>AFFTTVIIPAIVGGIATGTAVGTVSGLLGWGLKQAEEANKTPDKPDKVWRIQAGKGFNEFPNKEYDLYKSLLSSKIDGGWDWGNAATHYWIKGGQWNKLEVDMKDAVGTYKLSGLRNFTGGDLDVNMQKATLRLGQFNGNSFTSYKDSADRTTRVDFNAKNILIDNFLEINNRVGSGAGRKASSTVLTLQASEGITSSKNAEISLYDGATLNLASNSVKLNGNVWMGRLQYVGAYLAPSYSTINTSKVTGEVNFNHLTVGDHNAAQAGIIASNKTHIGTLDLWQSAGLNIIAPPEGGYKDKPNNTPSQSGAKNDKQESSQNNSNTQVINPPNSTQKTEVQPTQVIDGPFAGGKDTVVNIDRINTKADGTIKVGGFKASLTTNAAHLNIGKGGVNLSNQASGRTLLVENLTGNITVDGPLRVNNQVGGYALAGSSANFEFKAGVDTKNGTATFNNDISLGRFVNLKVDAHTANFKGIDTGNGGFNTLDFSGVTNKVNINKLITASTNVAVKNFNINELIVKTNGVSVGEYTHFSEDIGSQSRINTVRLETGTRSIFSGGVKFKSGEKLVIDEFYYSPWNYFDARNIKNVEITRKFASSTPENPWGTSKLMFNNLTLGQNAVMDYSQFSNLTIQGDFINNQGTINYLVRGGKVATLNVGNAAAMMFNNDIDSATGFYKPLIKINSAQDLIKNTEHVLLKAKIIGYGNVSTGTNGISNVNLEEQFKERLALYNNNNRMDTCVVRNTDDIKACGMAIGNQSMVNNPDNYKYLIGKAWKNIGISKTANGSK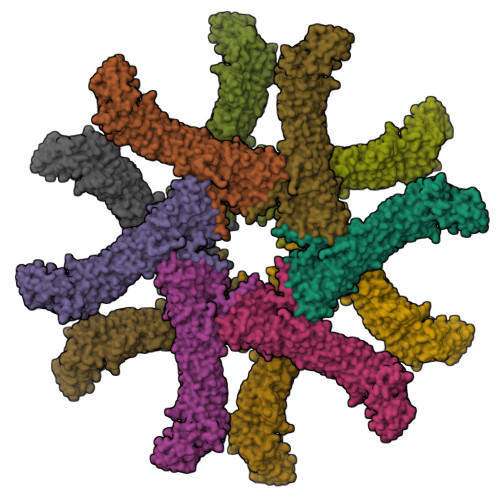ISVYYLGNSTPTENGGNTTNLPTNTTNNARFASYA[12x]> MRRTTGRAIAMAMLLALGQHAWAAACPGWAEGTAYKVGDVVSYNNANYTALVAHTAYVGANWNPAASPTLWTPGGS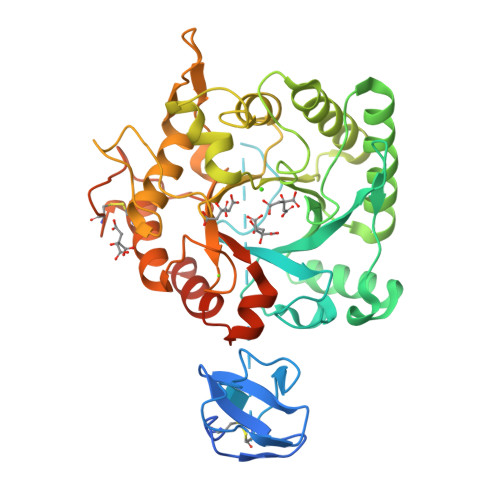CAGGDPTPPTPPNPPTPPSPPPGNTVPFAKHALVGYWHNFANPSGSAFPLSQVSADWDVIVVAFADDAGNGNVSFTLDPAAGSAAQFIQDIRAQQAKGKKVVLSLGGQNGSVTLNNATQVQNFVNSLYGILTQYGFDGIDLDLESGSGIVVGAPVVSNLVSAVKQLKAKIGPNFYLSMAPEHPYVQGGFVAYGGNWGAYLPIIDGLRDDLSVIHVQYYNNGGLYTPYSTGVLAEGSADMLVGGSKMLIEGFPIANGASGSFKGLRPDQVAFGVPSGRSSANSGFVTADTVAKALTCLTTLQGCGSVKPAQAYPAFRGVMTWSINWDRRDGYTFSRPVAASLRQQPVAAQAGKKKAARATRTAW> MDGSRGTAPGGDDLRGDRRDSYQGEDREDSHLLGALEDGNHQQSQGHGGGSGFYHHNVNSSSASVLEGVEMAHDELFAGPVAESVPTSVSAFSHRHGRAESVASFSFYHEQDDQREELEAPPGSLGARLSIDDLDELPFEEEGLSESEMPEQLDTFGIDLEWGSMNNGYPLIRRSSTHSQFSAHHRLLRRESGVSAASGYTGGRSSQKMRLDNDDLTIAISGFITNRIGFAIYIVLCVLTGGIAWLFLRWYPKYYVKLVGCATPFRDCQWVVIEDHFNKMTILSIRVKPYNRPLSTVFGTPSRATSWPLAQDPDPVLRELRSITYCYYKFYYHPVLDKFFCCNGWKDPQWNSMQNARSGLHGDEKAHREAVFGPNSIDVDEQSILQLLVSEILTPFYAFQVFSLI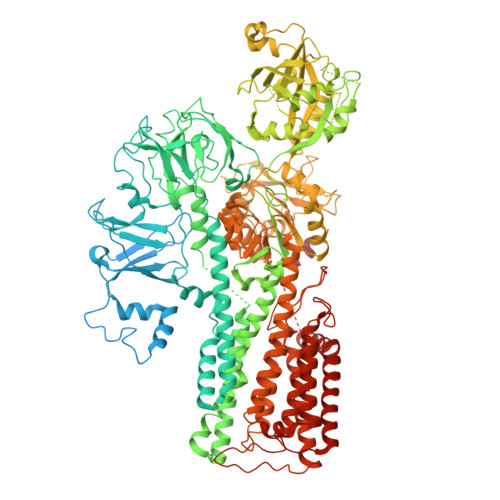LWLCDEYYYYAAAILLISAGSIITSLLETKETRRRLREMSRFECEVRVFRGGFWRTFPSSDLVPGDVYEVSDPSLTQIPADSLLLTGDCIVNESMLTGESVAVSKTPATNETLAKLNPAASTFSHDVDKHFLYCGTKLIRARQRLADTDEAAAVALVVRTGFNTTRGALVRSMLVPKPSKFKFYEDSFRYLKVMGCLAGLAFIVSLVNFIRLKLHWTLILLRALDLLTIVVPPALPATLTIGTSFAVQRLKGKKIFCTSPQRVNVGGKIDLMCFDKTGTLTEEGLDVLGIRVASRVSNRFTELLTNVDDLTWSCDSVSNGDEVKPADHVDGSSLKKDKTKPLDPYRAALYVMASCHSLRIVDGVAVGDPLEVKMFEFTGWSYEEGFIAGEVISTEGRGDISPSIARPPRYMTSQEMSIGEAPPAVGVLRAFDFNPLLRRSSVIARVVGNSGGYALVKGSPECMPEICRPETLPSDFDELLSYYTHAGYRVIACATKRIPKLNLVSVNRMTRDEVESGLDFVGFIIFENKLKPTTTSVIKELLSSNIGTVMITGDNIRTAVSVARQCGIIEEHAHCYMPRFIEGNADDCNAKLRWESINNPALELDPWTLLPMPVPPQTDASLPYDVSNIRNYAIAVTGDVFRWIVDHAPTDVLHRMLVLGKVYARMSPDEKQELVKKFQSIDYSCGFCGDGANDCAALKAADVGISLSEAEASVAAPFTSQIFDIRCVPEVIREGRASLVTSFSCFKYMSLYSFIQFTSVSFLYVSASNLGDFQFLYIDLMLILPIAVFMSWAGPHSKLCAKRPVSDLVSRKVLVPLLSHVFVCVMIQALAWVAVRQQPWYIPPIVDTEKSNIENSENTTLFFASCFEYILSGVVLNAGRPFRQSPLETWPFLSAVAVTLIATLLMLLVPPYWLFEFMQLTWMSWTFKITLIAFGFVYFLIAWTGEHYLFLWLARFLGRMRQRLFKQPKQRKLYKIVKEKLVF>GEGMWVPQQLPEIAGPLKKAGLKLSPQQISDLTGDPMGAVVALGGCTASFVSPNGLVVTNHACAYGAIQLNSTAENNLIKNGFNAPTTADEVSAGPNARVFVLDEITDVTKDAKAAIAAAGDDALARTKALEAFEKKLIADCEAEAGFRCRLYSFSGGNTYRLFKNLEIKDVRLAYAPPGSVGKFGGDIDNWMWPRHTGDFAFYRAYVGKDGKPAAFSKDNVPYQPKHWLKFADQPLGAGDFVMVAGYPGSTNRYALAAEFDNTAQWTYPTIARHYKNQIAMVEAAGKQNADIQVKYAATMAGWNNTSKNYDGQLEGFKRIDAAGQKLREEAAVLGWLKGQGAKGQPALDAHAKLLDLLEQSKATRDRDLTLALFNNTAMLGSATQLYRLSIEREKPNAERESGYQERDLPAIEGGLKQLERRYVAAMDRQLQEYWLNEYIKLPADQRVAAVDAWLGGNDAAAVKRALDRLAGTKLGSTEERLKWFAADRKAFEASNDPAIQYAVAVMPTLLKLEQERKTRAGENLAARPVYLQALADYKKSQGEFVYPDANLSLRITFGNVMGYAPKDGMEY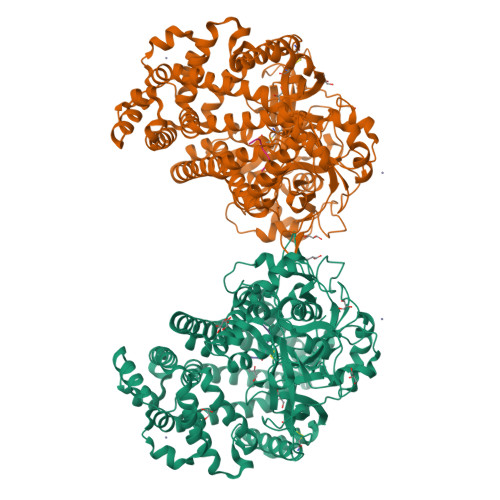TPFTTLEGVVAKETGQDPFDSPKALLDAVAAKRYGGLEDKRIGSVPVNYLSDLDITGGNSGSPVLDAHGKLVGLAFDGNWESVSSNWVFDPKMTRMIAVDGRYLRWIMQEVYPAPQLLKEMNVGK[2x];>VYIHPF[2x]>[4x]HHHHHHSSGLVPRGSHMASMSKVGINGFGRIGRLVLRRLLEVKSNIDVVAINDLTSPKILAYLLKHDSNYGPFPWSVDFTEDSLIVDGKSIAVYAEKEAKNIPWKAKGAEIIVECTGFYTSAEKSQAHLDAGAKKVLISAPAGEMKTIVYNVNDDTLDGNDTIVSVASCTTNCLAPMAKALHDSFGIEVGTMTTIHAYTGTQSLVDGPRGKDLRASRAAAENIIPHTTGAAKAIGLVIPELSGKLKGHAQRVPVKTGSVTELVSILGKKVTAEEVNNALKQATTNNESFGYTDEEIVSSDIIGSHFGSVFDATQTEITAVGDLQLVKTVAWYDNEYGFVTQLIRTLEKFAKL

Glyceraldehyde-3-phosphate dehydrogenase (GAPDH) is a highly conserved enzyme involved in the ubiquitous process of glycolysis and presents a loop (residues 208–215 of Escherichia coli GAPDH) in two alternative conformations (I and II). In the presence of inorganic phosphate (Pi), GAPDH catalyzes the conversion of D-glyceraldehyde-3-phosphate (G3P) to 1,3-diphosphoglycerate (BPG), accompanying the reduction of NAD+ to NADH. All the structures reported in this paper have four subunits: O, P, Q, and R. Each subunit contained two domains: the C-terminal catalytic domain and the N-terminal NAD+-binding domain. Two anion recognition sites, “Ps” and “Pi”, bind the C3 phosphate of G3P and inorganic phosphate, respectively.

The apparent KM value of the wild-type EcGAPDH1 enzyme for D-G3P was estimated to be 0.73 mM, the Vmax was 0.272 mM/min, and the Kcat was 224,926 min−1. The KM value of EcGAPDH1 was similar to that of Cryptosporidium parvum GAPDH (CpGAPDH). However, the Vmax was 171 times higher than that of CpGAPDH. This means that EcGAPDH1 may have a higher enzymatic activity than CpGAPDH. Amino acids Arg11, Ile12, Asp34, Arg78, Ser120, and Asn315, which form hydrogen bonds with NAD+, are highly conserved in WT and the mutant binary complex structure of EcGAPDH1. The overall structure analysis showed that the catalytic domain is an open pocket with positive charges.>MLVSVYLALLVACVGQAHSQANLMRLKSDLFNRSPMYPGPTKDDPLTVTLGFFLQDIVKVDSSTNEVDLVYYERQRWKLNSLMWDPNEYGNITDFRTSAADIWTPDITAASSTRPVQVLSPQIAVVTHDGSVMFSPAQRLSFMCDPTGVDSEEGVTCAVKFESWVYSGFEIDLKTDTDQVDLSSYYASSKYEILS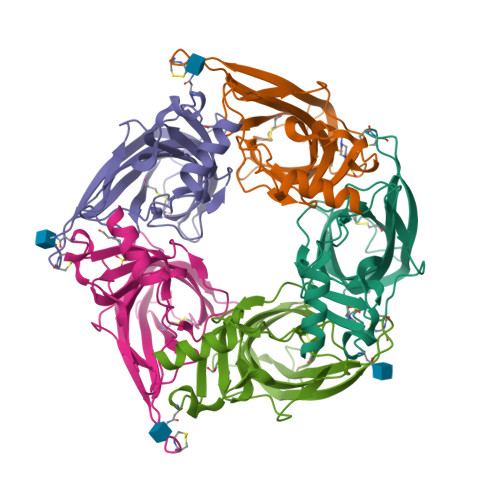ATQTRQVQHYSCCPEPYIDVNLVVKFRERRAGNGFFRNLFDENLYFQGHHHHHH[5x]>KKIFKPEELRQALMPTLEALYRQDPESLPFRQPVDPQLLGIPDYFDIVKNPMDLSTIKRKLDTGQYQ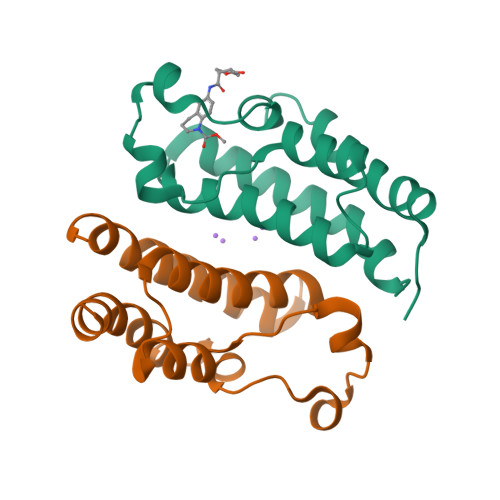EPWQYVDDVWLMFNNAWLYNRKTSRVYKFCSKLAEVFEQEIDPVMQSL[4x]>SNARTITYDVFLSFRGEDTRFNFTDHLYSALGRRGIRTFRDDKLRRGEAIAPELLKAIEESRSSVIVFSENYARSRWCLDALVKIMECHKDKKDPGHAVFPIFYHVDPSHVRKQEGSFGEAFAGYGENLKDKIPRWR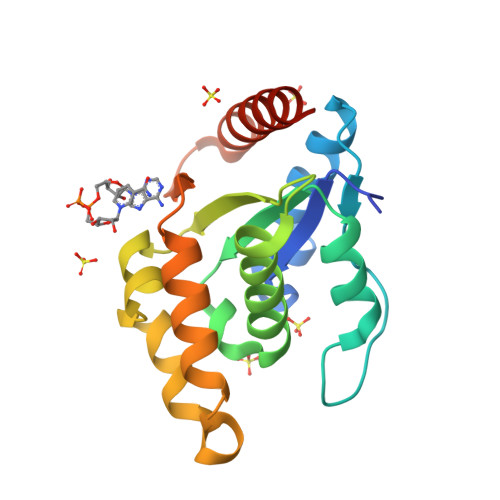TALTEAANLSGWPLQDGYESNQIKEITDSIFRRLKCKRLDAG[4x]>MGSSHHHHHHSQDPMGQVLPLVTRQGDRIAIVSGLRTPFARQATAFHGIPAVDLGKMVVGELLARSEIPAEVIEQLVFGQVVQMPEAPNIAREIVLGTGMNVHTDAYSVSRACATSFQAVANVAESLMAGTIRAGIAGGADSSSVLPIGVSKKLARVLVDVNKARTMSQRLKLFSRLRLRDLMPVPPAVAEYSTGLRMGDTAEQMAKTYGITREQQDALAHRSHQRAAQAWSDGKLKEEVMTAFIPPYKQPLVEDNNIRGNSSLADYAKLRPAFDRKHGTVTAANSTPLTDGAAAVILMTESRAKELGLVPLGYLRSYAFTAIDVWQDMLLGPAWSTPLALERAGLTMSDLTLIDMHEAFAAQTLANIQLLGSERFAREALGRAHATGEVDDSKFNVLGGSIAYGHPFAATGARMITQTLHELRRRGGGFGLVTACAAGGLGAAMVLEAE[4x];>[4x]MEMTSAFTLNVRLDNIAVITIDVPGEKMNTLKAEFASQVRAIIKQLRENKELRGVVFVSAKPDNFIAGADINMIGNCKTAQEAEALARQGQQLMAEIHALPIQVIAAIHGACLGGGLELALACHGRVCTDDPKTVLGLPEVQLGLLPGSGGTQRLPRLIGVSTALEMILTGKQLRAKQALKLGLVDDVVPHSILLEAAVELAKKERPSSRPLPVRERILAGPLGRALLFKMVGKKTEHKTQGNYPATERILEVVETGLAQGTSSGYDAEARAFGELAMTPQSQALRSIFFASTDVKKDPGSDAPPAPLNSVGILGGGLMGGGIAYVTACKAGIPVRIKDINPQGINHALKYSWDQLEGKVRRRHLKASERDKQLALISGTTDYRGFAHRDLIIEAVFENLELKQQMVAEVEQNCAAHTIFASNTSSLPIGDIAAHATRPEQVIGLHFFSPVEKMPLVEI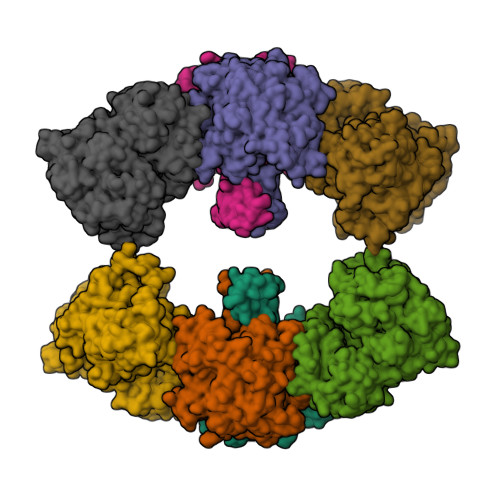IPHAGTSAQTIATTVKLAKKQGKTPIVVRDKAGFYVNRILAPYINEAIRMLTQGERVEHIDAALVKFGFPVGPIQLLDEVGIDTGTKIIPVLEAAYGERFSAPANVVSSILNDDRKGRKNGRGFYLYGQKGRKSKKQVDPAIYPLIGTQGQGRISAPQVAERCVMLMLNEAVRCVDEQVIRSVRDGDIGAVFGIGFPPFLGGPFRYIDSLGAGEVVAIMQRLATQYGSRFTPCERLVEMGARGESFWKTTATDLQ>[4x]MRGSHHHHHHGMASMPLHHLTRFPRLEFIGAPTPLEYLPRLSDYLGR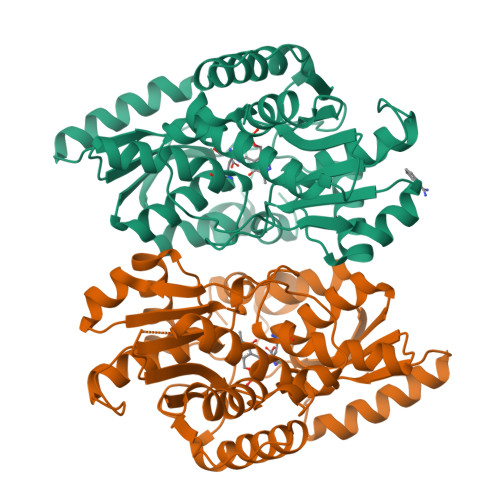EIYIKRDDVTPIAMGGNKLRKLEFLVADALREGADTLITAGAIQSNHVRQTAAVAAKLGLHCVALLENPIGTTAENYLTNGNRLLLDLFNTQIEMCDALTDPDAQLQTLATRIEAQGFRPYVIPVGGSSALGAMGYVESALEIAQQCEEVVGLSSVVVASGSAGTHAGLAVGLEHLMPDVELIGVTVSRSVAEQKPKVIALQQAIAGQLALTATADIHLWDDYFAPGYGVPNDAGMEAVKLLASLEGVLLDPVYTGKAMAGLIDGISQKRFNDDGPILFIHTGGAPALFAYHPHVTYPE>[10x]MAELPPGRLATTEDYFAQQAKQAVTPDVMAQLAYMNYIDFISPFYSRGCSFEAWELKHTPQRVIKYSIAFYAYGLASVALIDPKLRALAGHDLDIAVSKMKCKRVWGDWEEDGFGTDPIEKENIMYKGHLNLMYGLYQLVTGSRRYEAEHAHLTRIIHDE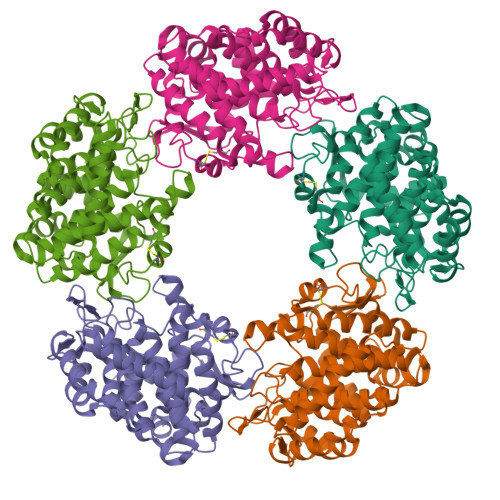IAANPFAGIVSEPDNYFVQCNSVAYLSLWVYDRLHGTDYRAATRAWLDFIQKDLIDPERGAFYLSYHPESGAVKPWISAYTTAWTLAMVHGMDPAFSERYYPRFKQTFVEVYDEGRKARVRETAGTDDADGGVGLASAFTLLLAREMGDQQLFDQLLNHLEPPAKPSIVSASLRYEHPGSLLFDELLFLAKVHAGFGALLRMPPPAAKLAGK Microbial ion-pumping rhodopsins (MRs) are extensively studied retinal-binding membrane proteins. The green-light absorbing proteorhodopsin (GPR) was originally discovered in marine γ-proteobacteria as the first bacterial rhodopsin and as an example of a new type of bacterial phototrophy. The bacterial green-light absorbing proton pump proteorhodopsin (GPR) has emerged as a model protein for MRs and is used here to address these open questions using cryo-electron microscopy (cryo-EM) and molecular dynamics (MD) simulations. GPR possesses an N-terminal signal sequence, akin to numerous membrane proteins, that is hypothesised to guide the correct insertion of the protein into the plasma membrane before subsequent proteolytic removal.

To this end, we expressed the GPR-A18L variant, introducing an alanine to leucine substitution (A18L) known to prevent cleavage of the signal peptide in the blue-light absorbing proteorhodopsin (BPR) when expressed in E. coli. Subsequent analysis of GPR-A18L oligomers by single particle cryo-EM revealed pentameric and hexameric particles. No corresponding densities were found in the pentameric GPR map. No density for the N-terminal signal peptides could be found, presumably due to significant flexibility and a lack of interactions. Conversely, if the signal peptides have moved away from the centre, the protomers can come into closer contact and form pentamers. In both the GPR-A18L pentamer and hexamer, the same two interaction areas are observed, comprising a large hydrophobic patch running along the membrane-embedded region and a polar interaction network towards the intracellular end. While most interactions involve the same residues, the hexameric GPR interface is slightly larger due to the closer proximity of the protomers and the narrower angle of encounter. This results in a larger surface area of 950 Å2 compared to 790 Å2 in the pentamer, excluding interfaces involving the signal peptide. Despite this increased contact area, nanoDSF analysis of isolated GPR-A18L pentamers and hexamers indicates greater stability of the pentamer. Using a GPR mutant with an uncleavable signal peptide, we solved the cryo-EM structures of pentameric and hexameric GPR, revealing that the signal peptide is involved in the formation of the GPR hexamer but not the pentamer.

>[5x]MGKLLLILGSVIALPTFLAGGGDLDASDYTGVSFWLVTAALLASTVFFFVERDRVSAKWKTSLTVSGLVTGIAFWHYMYMRGVWIETGDSPTVFRYIDWLLTVPLLICEFYLILAAATNVAGSLFKKLLVGSLVMLVFGYMGEAGIMAAWPAFIIGCLAWVYMIYELWAGEGKSACNTASPAVQSAYNTMMYIIIFGWAIYPVGYFTGYLMGDGGSALNLNLIYNLADFVNKILFGLIIWNVAVKESSNAGHHHHH>[38x]MRRNIFCLACLWIVQACLSLDRADILYNIRQTSRPDVIPTQRDRPVAVSVSLKFINILEVNEITNEVDVVFWQQTTWSDRTLAWNSSHSPDQVSVPISSLWVPDLAAYNAISKPEVLTPQLAHVVSDGEVQYTPSIRQRFSCDVSGVDTESGATCRIKIGSWTHHSREI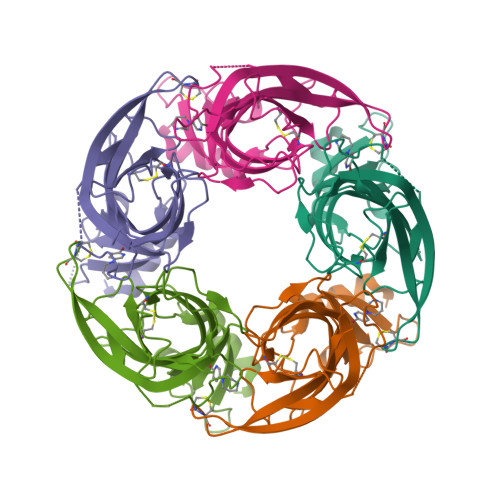SVDPTTENSDDSEYFSQYSRFEILDVTQKKNSVTYSCCPEAYEDVEVSLNFRKKGRSEIL;> MRRNIFCLACLWIVQACLSLDRADILYNIRQTSRPDVIPTQRRPVAVSVSLKFINILEVNEITNEVDVVFWQQTTWSDRTLAWNSSHSPDQVSVPISSLWVPDLAAYNAISKPEVLTPQLAHVVSDGEVQYTPSIRQRFSCDVSGVDTESGATCRIKIGSWTHHSREISVDPTTENSDDSEYFSQYSRFEILDVTQKKNSVTYSCCPEAYEDVEVSLNFRKKGRSEIL;> MRRNIFCLACLWIVQACLSLDRADILYNIRQTSRPDVIPTQRDRPVAVSVSLKFINILEVNEITNEVDVVFWQQTTWSDRTLAWNSSHSPDQVSVPISSLWVPDLAAYNAISKPEVLTPQLAHVVSDGEVQYTPSIRQRFSCDVSGVDTQSGATCRIKIGSWTHHSREISVDPTTENSDDSEYFSQYSRFEILDVTQKKNSVTYSCCPEAYEDVEVSLNFRKKGRSEIL>SADLAFEAKSARDYAWYDVSSFLTYRVLRTGE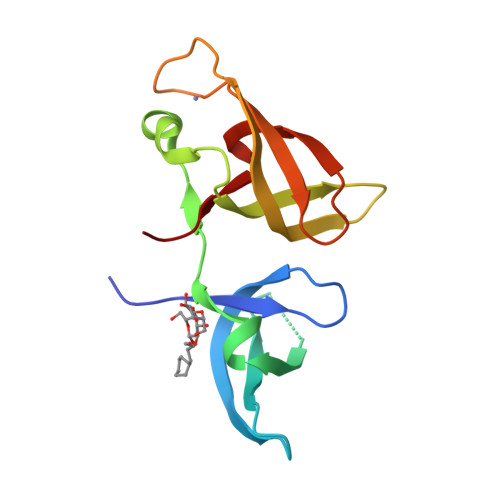LEVRVRFSGFDNRHDEWVNVKTSVRERSIPVEPSECGRVNVGDLLLCFQEREDQALYCDGHVLNIKRGIHDHARCNCVFLVRYELDNTEESLGLERICRRPEE[2x]> TA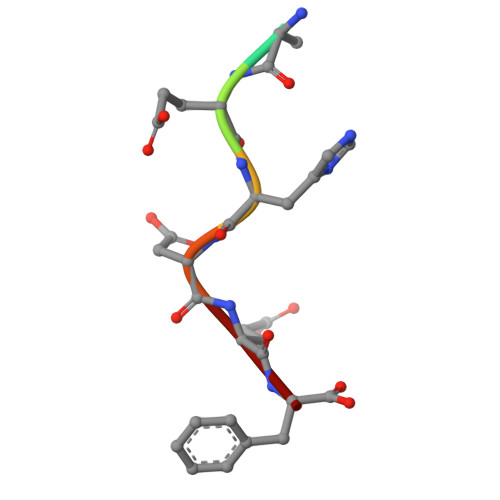EHDEF>SELQTEGRTRYHGRNVCSTWGNFHYKTFDGDVFRFPGLCDYNFASDCRGSYKEFAVHLKRGPGQAEAPAGVESILLTIKDDTIYLTRHLAVLNGAVVSTPHYSPGLLIEKSDAYTKVYSRAGLTLMWNREDALMLELDTKFRNHTCGLCGDYNGLQSYSEFLSDGVLFSPLEFGNMQKINQPDVVCEDPEEEVAPASCSEHRAECERLLTAEAFADCQDLVPLEPYLRACQQDRCRCPGGDTCVCSTVAEFSRQCSHAGGRPGNWRTATLCPKTCPGNLVYLESGSPCMDTCSHLEVSSLCEEHRMDGCFCPEGTVYDDIGDSGCVPVSQCHCRLHGHLYTPGQEITNDCEQCVCNAGRWVCKDLPCPGTCALEGGSHITTFDGKTYTFHGDCYYVLAKGDHNDSYALLGELAPCGSTDKQTCLKTVVLLADKKKNAVVFKSDGSVLLNQLQVNLPHVTASFSVFRPSSYHIMVSMAIGVRLQVQLAPVMQLFVTLDQASQGQVQGLCGNFNGLEGDDFKTASGLVEATGAGFANTWKAQSTCHDKLDWLDDPCSLNIESANYAEHWCSLLKKTETPFGRCHSAVDPAEYYKRCKYDTCNCQNNEDCLCAALSSYARACTAKGVMLWGWREHVCNKDVGSCPNSQVFLYNLTTCQQTCRSLSEADSHCLEGFAPVDGCGCPDHTFLDEKGRCVPLAKCSCYHRGLYLEAGDVVVRQEERCVCRDGRLHC[2x];>[2x]RQIRLIGQSCTAPKIHMDCSNLTALATSKPRALSCQTLAAGYYHTECVSGCVCPDGLMDDGRGGCVVEKECPCVHNNDLYSSGAKIKVDCNTCTCKRGRWVCTQAVCHGTCSIYGSGHYITFDGKYYDFDGHCSYVAVQDYCGQNSSLGSFSIITENVPCGTTGVTCSKAIKIFMGRTELKLEDKHRVVIQRDEGHHVAYTTREVGQYLVVESSTGIIVIWDKRTTVFIKLAPSYKGTVCGLCGNFDHRSNNDFTTRDHMVVSSELDFGNSWKEAPTCPDVSTNPEPCSLNPHRRSWAEKQCSILKSSVFSICHSKVDPKPFYEACVHDSCSCDTGGDCECFCSAVASYAQECTKEGACVFWRTPDLCPIFCDYYNPPHECEWHYEPCGNRSFETCRTINGIHSNISVSYLEGCYPRCPKDRPIYEEDLKKCVTADKCGCYVEDTHYP;>[2x]PGASVPTEETCKSCVCTNSSQVVCRPEEGKILNQTQDGAFCYWEICGPNGTVEKHFNICSITTRPSTLTTFTTITLPTTPTSFTTTTTTTTPTSSTVLSTTPKLCCLWSDWINEDHPSSGSDDGDRETFDGVCGA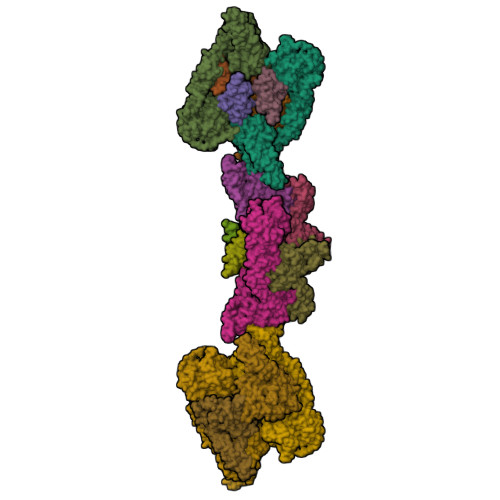PEDIECRSVKDPHLSLEQHGQKVQCDVSVGFICKNEDQFGNGPFGLCYDYKIRVNCCWPMDKCITHHHHHH3,4-PYRROLIDINEDIOL,2-(4-AMINO-5H-PYRROLO[3,2-D]PYRIMIDIN-7-YL)-5-(HYDROXYMETHYL)-2S,3S,4R,5R | C11 H15 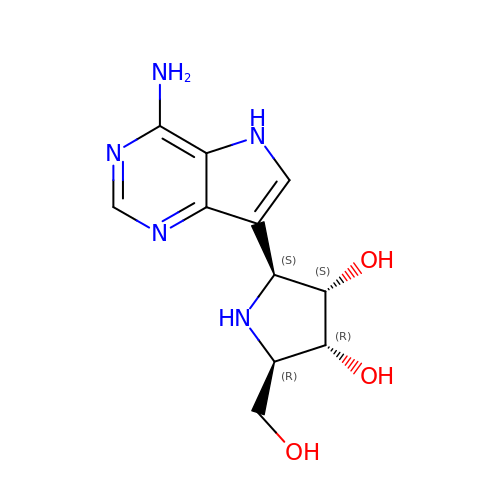N5 O3 | AMFDITJFBUXZQN-KUBHLMPHSA-N> YEYVELAKASLTSAQPQHFYAVVIDATFPYKTNQERYICSLKIVDPTLYLKQQKGAGDASDYATLVLYAKRFEDLPIIHRAGDIIRVHRATLRLYNGQRQFNANVFYSSSWALFSTDKRSVTQEINNQDAVSDTTPFSFSSKHATIEKNEISILQNLRKWANQYFSSY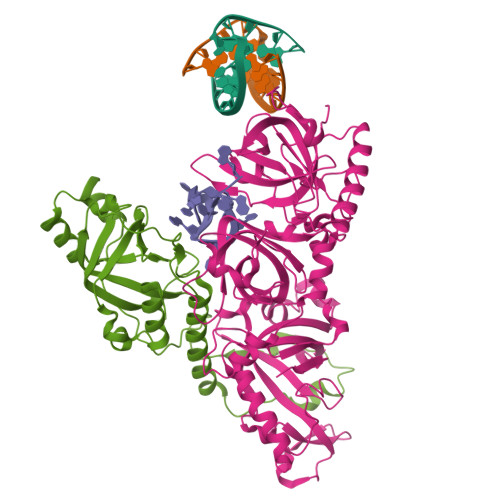SVISSDMYTALNKAQAQKGDFDVVAKILQVHELDEYTNELKLKDASGQVFYTLSLKLKFPHVRTGEVVRIRSATYDETSTQKKVLILSHYSNIITFIQSSKLAKELRAKIQDDHSVEVASLKKNVSLNAVVLTEVDKKHAALPSTSLQDLFHHADSDKELQAQDTFRTQFYVTKIEPSDVKEWVKGYDRKTKKSSSLKGASGKGDNIFQVQFLVKDASTQLNNNTYRVLLYTQDGLGANFFNVKADNLHKNADARKKLEDSAELLTKFNSYVDAVVERRNGFYLIKDTKLIY;> QQQSAFKQLYTELFNNEGDFSKVSSNLKKPLKCYVKESYPHFLVTDGYFFVAPYFTKEAVNEFHAKFPNVNIVDLTDKVIVINNWSLELRRVNSAEVFTSYANLEARLIVHSFKPNLQERLNPTRYPVNLFRDDEFKTTIQHFRHTALQAAINKTVKGDNLVDISKVADAAGKKGKVDAGIVKASASKGDEFSDFSFKEGNTATLKIADIFVQEKG>WDGKIDGTGTHAMIVTQGVSILENDLSKNEPESVRKNLEILKENMHELQLGSTYPDYDKNAYDLYQDHFWDPDIDNNFSKDNSWYLAYSIPDTGESQIRKFSALARYEWQRGNYKQATFYLGEAMHYFGDIDTPYHPANVTAVDSAGHVKFETFAEERKEQYKINTAGCKTNEAFYTDILKNKDFNAWSKEYARGFAKT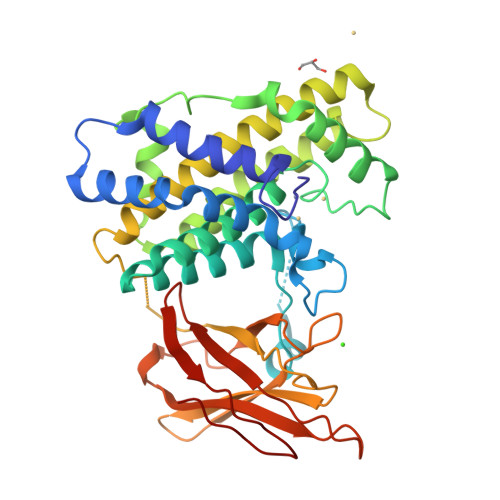GKSIYYSHASMSHSWDDWDYAAKVTLANSQKGTAGYIYRFLHDVSEGNDPSVGKNVKELVAYISTSGEKDAGTDDYMYFGIKTKDGKTQEWEMDNPGNDFMTGSKDTYTFKLKDENLKIDDIQNMWIRKRKYTAFPDAYKPENIKIIANGKVVVDKDINEWISGNSTYNIK[3x]> MEKTEKNELVRKLIFNPQGDREASKRKIIKGNPTNIFELNEIKYSWAFDLYKLMGFTNFWIPEEIQMLEDRKQYETVLSDYEKRAYELVLSFLIALDSFQVDMLKEFGRMITAPEVEMAITAQEFQESVHAYSYQFILESVVDPVKADEIYNYWREDERLLERNKVIAELYNEFIRKPNEENFIKATIGNYILESLYFYSGFAFFYTLGRQGKMRNTVQQIKYINRDELCHVTLFRNIINTLRKENPELFTPEIEKWIVEYFKYAVNEEIKWGQYVTQNQILGINDVLIERYIKYLGNLRITQIGFDPIYPEVTENPLKWIDEFRKINNTKTDFFQAKPQTYSKANELKW

pmcThe enzyme ribonucleotide reductase (RNR) synthesizes the deoxyribonucleotides needed for DNA synthesis from their corresponding ribonucleotide precursors. Class I RNRs are composed of two proteins, a large α-subunit (R1) and a smaller β-subunit (R2) that exist as homodimers, that combine to form an active heterotetramer. Aquifex aeolicus is a hyperthermophilic bacterium with an unusual RNR encoding a 346-residue intein in the DNA sequence encoding its R2 subunit. We present the first structures of the A. aeolicus R1 and R2 (AaR1 and AaR2, respectively) proteins as well as the biophysical and biochemical characterization of active and inactive A. aeolicus RNR.

Another possibility for the low radical content and poor occupancy for the second iron is that the presence of a reductant (TCEP) during purification may have partially reduced the tyrosyl radical and/or iron cluster. To address this, we purified AaR2 and AaR2_genomic again in the complete absence of reducing agent. We determined the X-ray crystal structures of TCEP free AaR2 and AaR2_genomic to resolutions of 2.15 and 2.10 Å, respectively. Superposition of AaR2 with AaR2_genomic (without TCEP) with their corresponding structures (with TCEP) shows the overall structures are virtually identical, with low RMSD values of 0.22 and 0.25 Å for the AaR2 and AaR2_genomic proteins, respectively. The AaR2_genomic structure (no TCEP) on the contrary showed clear electron density for both Fe1 and Fe2 in the active site. This is a significant improvement from the AaR2_genomic (with TCEP) structure, where the density for Fe2 was much weaker [modeled in at 0.25 occupancy]. The resulting crystal structures showed AaR2_genomic had full occupancy for both Fe1 and Fe2, indicating the presence of TCEP in the purification buffer was in fact affecting Fe2 binding during crystallization. TXRF analysis showed that AaR2_genomic consistently had a higher Fe content, and the activity was double that of AaR2, regardless of whether or not the proteins were purified with a reducing agent. This clearly shows that the intein in AaR2_genomic enhances the incorporation of iron into the mature protein, particularly in the Fe2 site.>MVNVEEIRKAQRAEGPAAILAIGTATPPNAIEQSEYPDYYFRVTNSEDKVELKEKFKRMCEKSMIKKRYLYLTEDILKENPNVCAYMATSLDARQDMVVVEVPKLGKEAATRAIKEWGQPKSKITHLVFCTTSGVDMPGADYQLTKLLGLRPSVKRLMMYQQGCFAGGTVLRLAKDLAENNRGARVLVVCSEITAVTFRGPSESHLDSLVGQALFGDGAAALIVGSDAIEGIERPIFEMVSAAQTILPDSEGAIDGHLREVGLTFHLLKDVPGIISKNIEKSLEEAFKPLGITDYNSLFWIAHPGGPAILDQVEAKIGLKPEKLRATRHVLSEYGNMSSACVLFILEEMRKKSAEEKNGTTGEGLEWGVLFGFGPGLTVETVVLHSVEA[4x]

CHS, the best studied plants-specific type III ployketide synthase, catalyses the first committed step of the branch of the phenylpropanoid pathway which leads to the synthesis of flavonoids. Enzymes of the CHS superfamily share high similarity in their amino acid sequence, structure and general catalytic principles and function as a homodimer (monomer size about 43 kDa) which contains the conserved Cys-His-Asn catalytic triad in the buried active sites. Briefly, the biosynthesis of flavonoid starts with the condensation of one molecule of p-coumaroyl-CoA (derived from the general phenylpropanoid pathway) with three molecules of malonyl-CoA, resulting in naringenin chalcone and this reaction is conducted by chalcone synthase (CHS). Furthermore, a previous study also showed that the reaction catalyzed by CHS can be seen as a three-step reaction which involves transfering the p-coumaroyl moiety to the active site residue Cys164, decarboxylation of malonyl-CoA to an acetyl-CoA carbanion and extending the polyketide intermediate.

In conclusion, we have successfully isolated FhCHS1, a CHS gene from Freesia hybrida, and examined its biological function in flavonoid biosynthesis. The gene has one intron with an open reading frame of 1,170 bp encoding 389 amino acid residues with a calculated molecular mass of 42.58 kDa and an isoelectric point of 5.74. Multiple sequence alignments revealed that FhCHS1 shared 83.55% to 85.86% identity with AtCHS, PhCHS and MsCHS2. Consistent with previous results with other CHS proteins, the FhCHS1 protein also contained the three important catalytic residues of Cys164, His303, and Asn336 (marked with pink background) and two highly conserved Phe residues, Phe215 and Phe265 (marked with blue background), which were identified to be important for the formation of the active site as well as for the substrate specificity of the CHS. Additionally, the malonyl-CoA binding motif (marked with yellow background) and a highly conserved CHS signature sequence (marked with red background) were also found in the FhCHS1 sequence. As shown in Fig. 2B&C, the crystallographic symmetry of FhCHS1 is a dimer of dimer, with the homodimer as the biological functional unit. The individual monomer consists of roughly two domains with the active site located at the clef between the two domains and the dimerization interface, therefore sharing the accessible substrate binding area with the dimer partner. Protein sequence alignment and structure analysis indicated the strong conservation of the sequence and structure of CHS protein, and these results provided some evidence for its enzymatic function. Compared with control, the reaction product generated a new peak at a retention time (28.5 min) that matched the authentic naringenin. This indicates that FhCHS1 has a typical CHS enzymatic function, catalyzing the conversion of p-coumaroyl-CoA and malonyl-CoA substrates to naringenin chalcone.> MIVSDIEANALLESVTKFHCGVIYDYSTAEYVSYRPSDFGAYLDALEAEVARGGLIVFHNGHKYDVPALTKLAKLQLNREFHLPRENCIDTLVLSRLIHSNLKDTD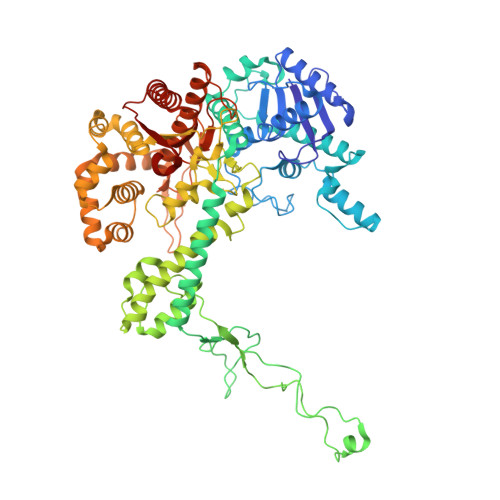MGLLRSGKLPGKRFGSHALEAWGYRLGEMKGEYKDDFKRMLEEQGEEYVDGMEWWNFNEEMMDYNVQDVVVTKALLEKLLSDKHYFPPEIDFTDVGYTTFWSESLEAVDIEHRAAWLLAKQERNGFPFDTKAIEELYVELAARRSELLRKLTETFGSWYQPKGGTEMFCHPRTGKPLPKYPRIKTPKVGGIFKKPKNKAQREGREPCELDTREYVAGAPYTPVEHVVFNPSSRDHIQKKLQEAGWVPTKYTDKGAPVVDDEVLEGVRVDDPEKQAAIDLIKEYLMIQKRIGQSAEGDKAWLRYVAEDGKIHGSVNPNGAVTGRATHAFPNLAQIPGVRSPYGEQCRAAFGAEHHLDGITGKPWVQAGIDASGLELRCLAHFMARFDNGEYAHEILNGDIHTKNQIAAELPTRDNAKTFIYGFLYGAGDEKIGQIVGAGKERGKELKKKFLENTPAIAALRESIQQTLVESSQWVAGEQQVKWKRRWIKGLDGRKVHVRSPHAALNTLLQSAGALICKLWIIKTEEMLVEKGLKHGWDGDFAYMAWVHDEIQVGCRTEEIAQVVIETAQEAMRWVGDHWNFRCLLDTEGKMGPNWAICH>GSHMASPNGQTKPLPALKLALEYIVPCMNKHGICVVDDFLGKETGQQIGDEVRALHDTGKFTDGQLVSQKSDSSKDIRGDKITWIEGKEPGCETIGLLMSSMDDLIRHCNGKLGSYKINGRTKAMVACYPGNGTGYVRHVDNPNGDGRCVTCIYYLNKDWDAKVSGGILRIFPEGKAQFADIEPKFDRLLFFWSDRRNPHEVQPAYATRYAITVWYFD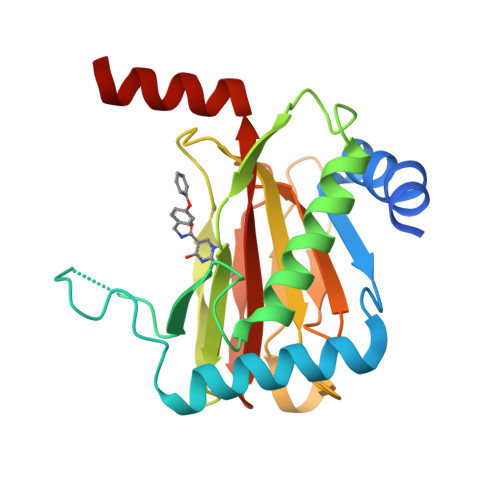ADERARAKVKYLTGE[2x]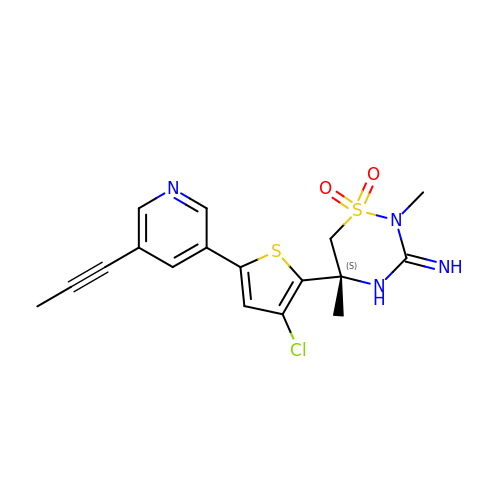(3E,5S)-5-{3-chloro-5-[5-(prop-1-yn-1-yl)pyridin-3-yl]thiophen-2-yl}-2,5-dimethyl-1,2,4-thiadiazinan-3-imine 1,1-dioxide | C17 H17 Cl N4 O2 S2 | VKVMIZCLMUKTTA-KRWDZBQOSA-N>[28x]ALVPMVIEQTSRGERSFDIYSRLLKERVIFL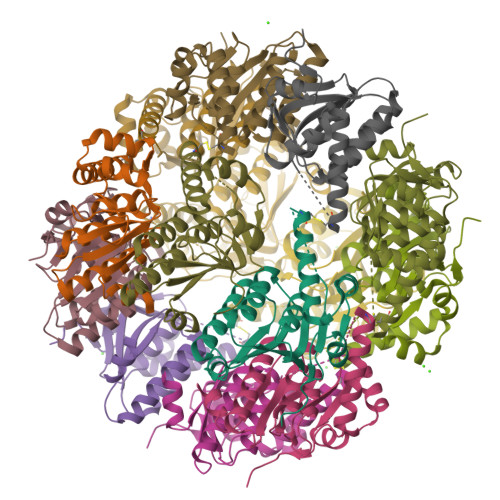TGQVEDHMANLIVAQMLFLEAENPEKDIYLYINSPGGVITAGMSIYDTMQFIKPDVSTICMGQAASMGAFLLTAGAKGKRFCLPNSRVMIHQPLGGYQGQATDIEIHCREILKVKGRMNELMALHTGQSLEQIERDTERDRFLSAPEAVEYGLVDSILTHRN>RPASTTLPAGADLADRFAELERRYDARLGVYVPATGTTAAIEYRADERFAFCSTFKAPLVAAVLHQNPLTHLDKLITYTSDDIRSISPVAQQHVQTGMTIGQLCDAAIRYSDGTAANLLLADLGGPGGGTAAFTGYLRSLGDTVSRLDAEEPELNRDPPGDERDTTTPHAIALVLQQLVLGNALPPDKRALLTDWMARNTTGAKRIRAGFPADWKVIDKTGTGDYGRANDIAVVWSPTGVPYVVAVMSDRAGGGYDAEPREALLAEAATCVAGVLA[4x]

In line with this proposal, the genome of M. tuberculosis harbors a chromosomal class A (Ambler) β-lactamase encoded by blaC. The efficiency with which BlaC thwarts β-lactam chemotherapy stems from its ability to hydrolyze penicillin, cephalosporin, and carbapenem classes of β-lactams. BlaC is a 307-amino-acid protein that bears an N-terminal Tat signal peptide and is natively exported by the Tat pathway in mycobacteria. When blaC was deleted from M. tuberculosis, the resulting cells exhibited increased susceptibility to β-lactam antibiotics by 8- to 256-fold, thereby linking BlaC with the intrinsic resistance to β-lactam chemotherapy.

Given that earlier BlaC crystal structures were for a truncated version of the enzyme that lacked the first 40 amino acids, we decided to crystallize the full-length version of the enzyme. Crystals were present in the P21 space group, and diffraction data to 2.8 Å resolution were used to solve the final structure with molecular replacement methods and the structure of the truncated BlaC enzyme. Despite the inclusion of the authentic N-terminal residues, the overall structure of full-length BlaC is very similar to the previously solved structure for truncated BlaC, a monomer containing an α domain and an α/β domain. Previous sequence alignment of BlaC with other known class A β-lactamases revealed that the region 102IRSISP107 of M. tuberculosis BlaC, which harbors the I105F substitution, is quite different from other class A β-lactamases. Whereas most other class A β-lactamases have either tyrosine or histidine with their aromatic side chains covering the entrance to the active site, Ile105 at the same position makes BlaC’s active site 3 Å wider than other class A β-lactamases. Interestingly, our I105F substitution reintroduces an aromatic side chain in this position. While we were unable to solve the structure for BlaC(I105F), the structural impact of this substitution in the context of the neighboring BlaC residues was investigated by modeling the I105F substitution in the wt BlaC structure. Specifically, we found that the measured distance from Ile105 to a nearby active site residue was 6.7 Å whereas the distance from the modeled Phe105 mutation to the same nearby residue was 10.3 Å, signifying a significant increase in the opening of the mutant enzyme’s active site compared to the parental enzyme. Further structural alignment of the computationally modeled I105F mutant with both wt BlaC and TEM-1 Bla revealed that the mutant’s active site more closely resembles that of TEM-1 Bla, with the Phe105 mutation aligning closely with an active site Tyr residue of TEM-1 Bla. While this structural model is insufficient to unequivocally establish how this mutation improves catalytic efficiency, it suggests that Ile105 of BlaC may function as a ‘gatekeeper’ residue that regulates substrate accessibility to the enzyme active site.>[2x]GSHMNGPIIMTREERMKIVHEIKERILDKYGD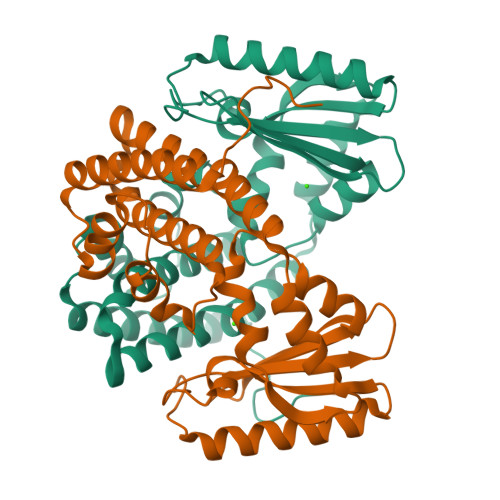DVKAIGVYGSLGRQTDGPYSDIEMMCVMSTEEAEFSHEWTTGEWKVEVNFDSEEILLDYASQVESDWPLTHGQFFSILPIYDSGGYLEKVYQTAKSVEAQKFHDAICALIVEELFEYAGKWRNIRVQGPTTFLPSLTVQVAMAGAMLIGLHHRICYTTSASVLTEAVKQSDLPSGYDHLCQFVMSGQLSDSEKLLESLENFWNGIQEWTERHGYIVDVSKRIPF2-{4-[2-ACETYLAMINO-2-(1-BIPHENYL-4-YLMETHYL-2-OXO-AZEPAN-3-YLCARBAMOYL)-ETHYL]-2-METHOXYCARBONYL-PHENYL}-2-FLUORO-MALONIC 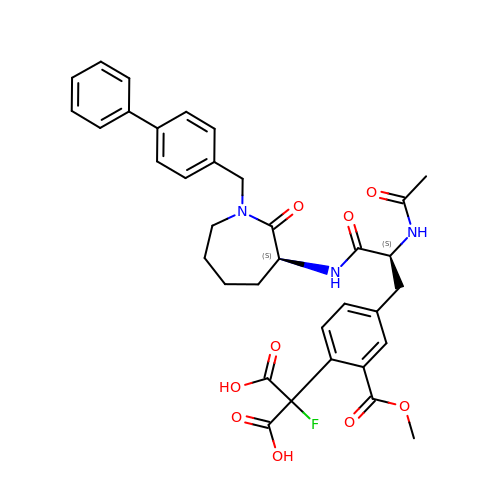ACID | C35 H36 F N3 O9 | RLLAUERCSKPFGD-VMPREFPWSA-N> GPGSPYGQQPQN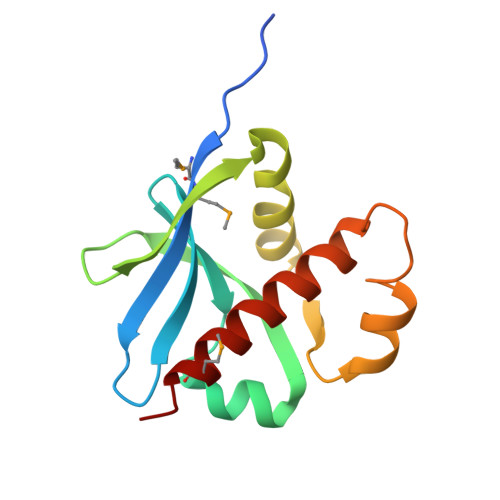RMMKLAYLDRGFYKHYGIIVGDHVYQLDSDDIFKTALTGKAKFTKTKLTSDWVIEEECELDYFRIKYLESAVDSEHIFSVDKNCETIAKDIFGTHTLSQHQAIGLVGTILLTAGLMSTIK> GPHMPGSGQIQLWQFLLELLSD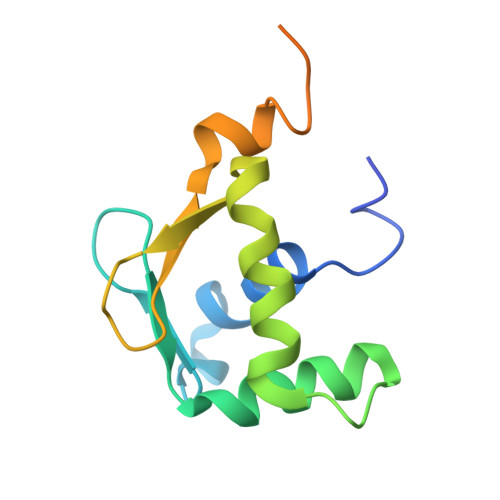SSNSSCITWEGTNGEFKMTDPDEVARRWGERKSKPNMNYDKLSRALRYYYDKNIMTKVHGKRYAYKFDFHGIAQALQPHPPESSLYKYPSDLPYMGSYHAHPQKMN> KKRYDREFL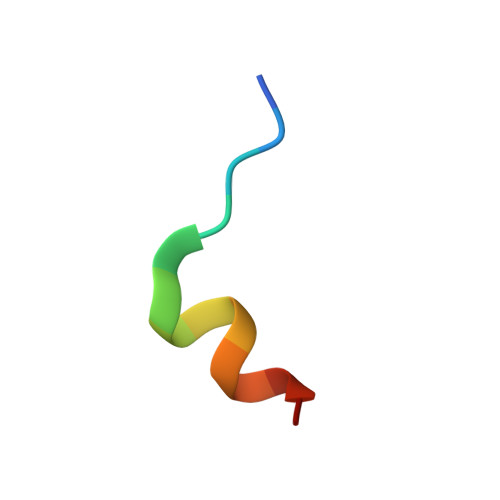LGFQF>[2x]GLTIGTHLIPHPRKAETGGEDAFFVNGDDGGVFAVADGVSGWAEKDVNPALFSRELMAHTSTFLKDEEVNHDPQLLLMKAHAATTSVGSATVIIAMLEKTG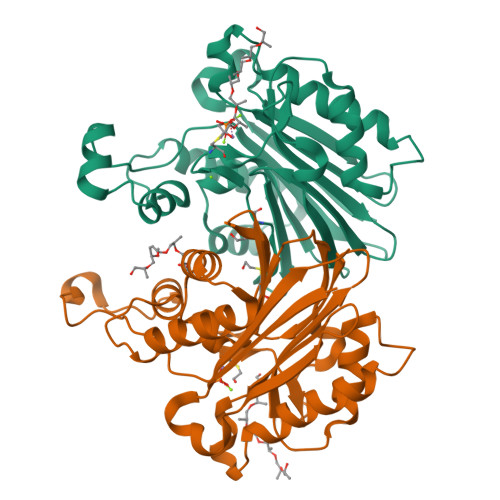ILKIASVGDCGLKVIRKGQVMFSTCPQEHYFDCPYQLSSEAIGQTYLDALVCTVNLMEGDMIVSGSDGFFDNIFDQEIVSVISESPGVDEAAKALAELARKHSVDVTFDSPYSMEARSRGFDVPSWKKFIGGKLIGGKMNDITVIVAQVKALEHHHHHH> GPFTMDNKSAVSALQEFCARTQINLPTYSFIPGE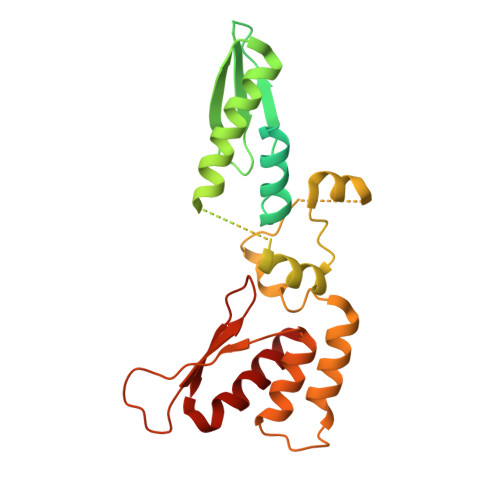DGGYVCKVELLEIEALGNGRSKRDAKHLAASNILRKIQLLPGIHGLMKDSTVGDLDEELTNLNRDMVKELRDYCVRREMPLPCIEVVQQSGTPSAPEFVACCSVASIVRYGKSDKKKDARQRAAIEMLALISSNSDNLRPDQMQVASTSKLKVVDMEESMEELEALRRKKFTTYWELKEAGSVDHTGMRLCDRHNYFKNFYPTLKKEAIEAINSDEYESSKDKAMDVMSSLKITPKISEVESSSLVPLLSVELNCAFDVVLMAKETDIYDHIIDYFRTMLI> ASMTGGQQMGRGSASLPACPEESPLLVGPMLIEFNMPVDLELVAKQNPNVKMGGRYAPRDCVSPHKVAIIIPFRNRQEHLKYWLYYLHPVLQRQQ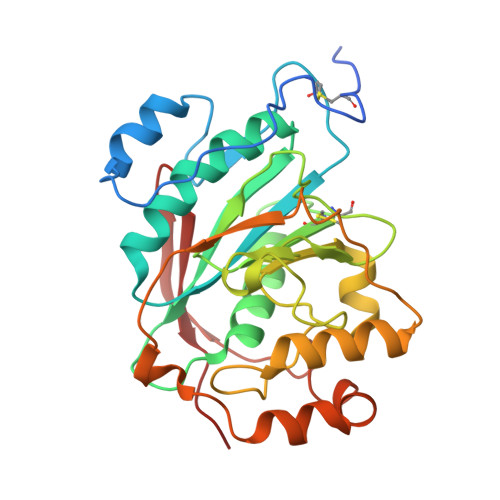LDYGIYVINQAGDTIFNRAKLLNVGFQEALKDYDYTCFVFSDVDLIPMNDHNAYRCFSQPRHISVAMDKFGFSLPYVQYFGGVSALSKQQFLTINGFPNNYWGWGGEDDDIFNRLVFRGMSISRPNAVVGTTRMIRHSRDKKNEPNPQRFDRIAHTKETMLSDGLNSLTYQVLDVQRYPLYTQITVDIGTPS>GAMGSGIQMKEEASEHGGSADETQELSPVSDSSDEMPNNAKRRRRSQSMIANKRIHQAFQEDEGDEDWEEEEHKPKAKRRYNTRSNESFSEGDDEPFEVSESSALEDELSDSEDSFIRSVRSKPKYKPGTRRSTRLRNRRSQDEEESEEEHRPILRERTSRINYSVPLAFPPVDEMDGDPSSQVNQSRSRKTHSELAITKLLRQQVSSFMPYIDSSGSESESDNTRIKKSSAKTIKALTDPANSGGPPDFGRIREKSDLADSDPLGVDSSLSFESVGGLDNYINQLKEMVMLPLLYPEIFQRFNMQPPRGVLFHGPPGTGKTLMARALAAACSSENKKVSFYMRKGADCLSKWVGEAERQLRLLFEEAKSTQPSIIFFDEIDGLAPVRSSKQEQIHASIVSTLLALMDGMESRGQVIIIGATNRPDAVDPALRRPGRFDREFYFPLPDRDARKKIIEIHTRNWDPPVPEWLCSMLAEKSKGYGGADLRALCTEAALNSIKRTYPQLYRSTKRLQIDPKTIKVKVKDFVMSMKRMIPSSERSSISPSKPLSPELKPLLNEAFQDIEKTLQKLMPVASKLNPLEEVMYDDPKENDFEYQQRLETFETLRIYKPRFLICGRKGLGQTALGPAILQQYEGVHVQSFDMSTLLQDSTQSIETSIIHLFLEVRRHTPSIIYIPDIDNWLNVLPLTAITTFSSMLERLDFSDQILFLALSSSPLSELHPQLREWFSSKQSVYSLQYPTRDSIIAFFQPILELIKASPTELPGGIPRKRRVLPELPLAPDPPPFTSQKITLKQTKQADMRLLNKLKIKLNALLGSLRARYRKFKKPLIDFNDIYCVDPETGHSYRSREECHYEFVDDVVKQIGSDQKFSMMSLEEIEKRTWDNCYCTPKQFVHDIKLILRDALQLEDSETIKRAQEMYANVLLGVEDMEDDQFSQRCERMALREAERRKLRHGKLQKHLDETKADMQFTSEKPSVDESITEVDDAIKDGPPVLAETLTNSLMEDVGPENVDMDIEDNEIFTNQSTMSVPSMLVENEESPKPDEYIDQKDKVQSPLLNGKSPVGVPSEAALRVSTDVSTNISSNGRADIPVDTLITSPADVPNNAPTDAHNITSADGHIENIEQEVVFPDLVFDEDRLTPLKQLLIDSTTGFTVDQLLHLHSFLYQIIWNTKSEWNRNSVVDECERAVKEFMINALQ[6x]

ATAD2 (also termed ANCCA) is a histone chaperone that has been implicated in nucleosome density regulation by histone H3–H4 loading or removal. Although histone chaperones responsible for nucleosome assembly and disassembly usually do not contain ATPase domains, ATAD2 is unique because it is the only known AAA+ ATPase histone chaperone. Here, we demonstrate ATP-dependent histone H3–H4 deposition onto DNA by Abo1, the fission yeast ortholog of ATAD2, using an in vitro single-molecule imaging technique, the DNA curtain. We solve the cryo-EM structures of Abo1 in three different nucleotide states (apo, ADP, and ATP), revealing a major reorganization of the AAA+ domains from an open spiral to a closed ring—a structural change that can also be recapitulated in real time by high-speed atomic force microscopy (HS-AFM).

To dissect nucleotide-dependent structural changes of Abo1, we next determined the cryo-EM structure of Abo1 in the ADP state to 4.4 Å resolution. We then performed flexible fitting of the ATP-model into the ADP- and apo- cryo-EM maps with MDFF16. Comparison of the ATP-Abo1 Walker B mutant structure with the ADP- and apo-states revealed striking differences in the subunit arrangement, heights and individual subunit conformation, while the structures of the ADP- and apo-states were similar to each other. In the ADP state, the subunits assumed similar heights forming a symmetric planar ring, whereas in the ATP-state, the subunits were staggered in height and shifted towards the center forming an asymmetric spiral with a smaller pore. The most prominent structural change could be observed at the interface of subunits A and F where in the ADP state, these two subunits maintained similar heights with close inter-subunit packing, while in the ATP state, the subunits were staggered in height and separated by ~40 Å. Individual subunits in the ADP state did not show any significant differences in their structures, supporting the idea that ADP-Abo1 is largely symmetric. When comparing the two extreme conformations of subunits (subunit A and subunit F) in the ATP-bound structure with the conformation of the subunit in the ADP-bound structure, we found that the bottom-most subunit in the ATP-bound structure (subunit A) superimposed well with the subunit in the ADP-bound structure, while the top-most subunit (subunit F) diverged significantly from the ADP-conformation. Lastly, but more interestingly, in contrast to the ATP-Abo1 structure, the bromodomain density was stronger and more symmetric in the ADP- and apo- structures. When ATP hydrolysis occurs, Abo1 transitions to a planar ring with a larger pore, potentially allowing for remodeling and/or release of histone H3–H4.>MEKNMKFPVVDLSKLNGEERDQTMALINEACENWGFFEIVNHGLPHDLMDKIEKMTKDHYKTCQEQKFNDMLKSKGLDNLETEVEDVDWESTFYVRHLPQSNLNDISDVSDEYRTAMKDFGKRLENLAEDLLDLLCENLGLEKGYLKKVFHGTKGPTFGTKVSNYPPCPKPEMIKGLRAHTDAGGIILLFQDDKVSGLQLLKDGDWIDVPPLNHSIVINLGDQLEVITNGKYKSVLHRVVTQQEGNRMSVASFYNPGSDAEISPATSLVEKDSEYPSFVFDDYMKLYAGVKFQPKEPRFAAMK[8x]

ACC is then oxidized by the ACC oxidase (ACCO or ACO, referred to as ACO in this study), giving rise to ethylene, carbon dioxide (CO2) and cyanide3. ACO enzyme is a 2OG-oxygenase ‘related' enzyme that belongs to the cupin superfamily, which uses a non-heme ferrous iron (Fe2+) as a cofactor and facilitates the integration of molecular oxygen into a myriad of biomolecules. ACO uses ascorbate, rather than 2-oxoglutarate as the co-substrate, and requires CO2, one of the products of the ACO reaction, as an activator. Overall, the structure of AtACO2 resembles the Petunia hybrid ACO (PhACO), featuring a double-stranded-helix jellyroll fold surrounded by α-helices.

Among the compounds tested, only 2-picolinic acid (2-PA) directly inhibited the enzymatic activity of AtACO2 like POA. Notably, the inhibition effect of 2-PA was stronger than that of POA, while a known ACO inhibitor, AIB, showed much weaker inhibition effect than POA in our assay. The SAR analyses identified 2-PA as an even more efficient inhibitor than POA. In the presence of Zn2+, POA and 2-PA bound to AtACO2 with dissociation constants (KD) of 10.2 and 2.8 μM, respectively. We subsequently co-crystallized AtACO2 with POA or 2-PA in the presence of Zn2+, and determined both structures at 2.1 Å. POA and 2-PA bind to AtACO2 in a similar manner. In both structures, the Zn2+ ion is coordinated by the facial triad, including His180, Asp182 and His237, and binds at a similar position as Fe2+ in PhACO. POA or 2-PA in turn binds to the Zn2+ via the carboxylate group and the N-2 nitrogen in the pyrazine or pyridine ring. The carboxylate group of POA or 2-PA forms a polar interaction with the side chain of Lys161. Lys291 contributes to the hydrogen bond interactions with POA or 2-PA through a water molecule.>GSHMASAARLTMMWEEVTCPICLDPFVEPVSIECGHSFCQECISQVGKGGGSVCPVCRQRFLLKNLRPNRQLANMVNNLKEISQEAREGTQGERCAVHGERLHLFCEKDGKALCWVCAQSRKHRD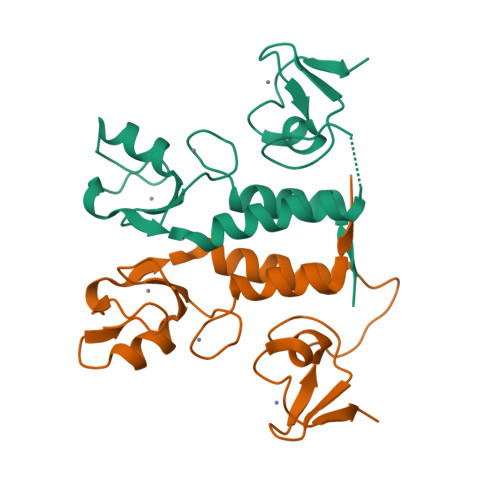HAMVPLE[2x]> MFIRIKCFSKQPIAKKVSREVSAYLEYTGNNTWEGHISGQGVSNLQTK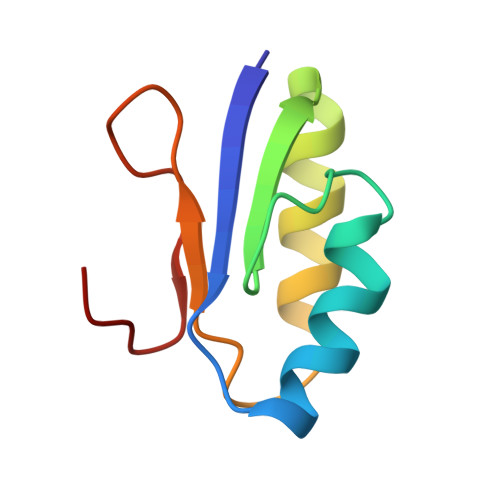LINVGKGVKVVCNYQDKVLFAIGNVAM>[2x]MEELQDDYEDMMEENLEQEEYEDPDIPESQMEEPAAHDTEATATDYHTTSHPGTHKVYVELQELVMDEKNQELRWMEAARWVQLEENLGENGAWGRPHLSHLTFWSLLELRRVFTKGTVLLDLQETSLAGVANQLLDRFIFEDQIRPQDREELLRALLLKHSHAGELEALGGVKPAVLTRSGDPSQPLLPQHSSLETQLFCEQGDGGTEGHSPSGILEKIPPDSEATLVLVGRADFLEQPVLGFVRLQEAAELEAVELPVPIRFLFVLLGPEAPHIDYTQLGRAAATLMSERVFRIDAYMAQSRGELLHSLEGFLDCSLVLPPTDAPSEQALLSLVPVQRELLRRRYQSSPAKPDSSFYKGLDLNGGPDDPLQQTGQLFGGLVRDIRRRYPYYLSDITDAFSPQVLAAVIFIYFAALSPAITFGGLLGEKTRN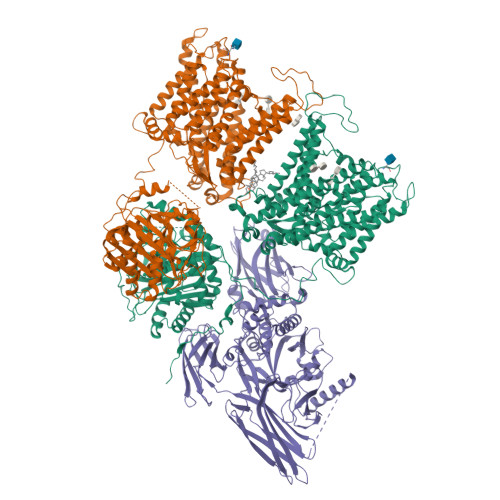QMGVSELLISTAVQGILFALLGAQPLLVVGFSGPLLVFEEAFFSFCETNGLEYIVGRVWIGFWLILLVVLVVAFEGSFLVRFISRYTQEIFSFLISLIFIYETFSKLIKIFQDHPLQKTYNYNVLMVPKPQGPLPNTALLSLVLMAGTFFFAMMLRKFKNSSYFPGKLRRVIGDFGVPISILIMVLVDFFIQDTYTQKLSVPDGFKVSNSSARGWVIHPLGLRSEFPIWMMFASALPALLVFILIFLESQITTLIVSKPERKMVKGSGFHLDLLLVVGMGGVAALFGMPWLSATTVRSVTHANALTVMGKASTPGAAAQIQEVKEQRISGLLVAVLVGLSILMEPILSRIPLAVLFGIFLYMGVTSLSGIQLFDRILLLFKPPKYHPDVPYVKRVKTWRMHLFTGIQIICLAVLWVVKSTPASLALPFVLILTVPLRRVLLPLIFRNVELQCLDADDAKATFDEEEGRDEYDEVAMPV;> MGQALGIKSCDFQAARNNEEHHTKALSSRRLFVRRGQPFTIILYFRAPVRAFLPALKKVALTAQTGEQPSKINRTQATFPISSLGDRKWWSAVVEERDAQSWTISVTTPADAVIGHYSLLLQVSGRKQLLLGQFTLLFNPWNREDAVFLKNEAQRMEYLLNQNGLIYLGTADCIQAESWDFGQFEGDVIDLSLRLLSKDKQVEKWSQPVHVARVLGALLHFLKEQRVLPTPQTQATQEGALLNKRRGSVPILRQWLTGRGRPVYDGQAWVLAAVACTVLRCLGIPARVVTTFASAQGTGGRLLIDEYYNEEGLQNGEGQRGRIWIFQTSTECWMTRPALPQGYDGWQILHPSAPNGGGVLGSCDLVPVRAVKEGTLGLTPAVSDLFAAINASCVVWKCCEDGTLELTDSNTKYVGNNISTKGVGSDRCEDITQNYKYPEGSLQEKEVLERVEKEKMEREKDNGIRPPSLETASPLYLLLKAPSSLPLRGDAQISVTLVNHSEQEKAVQLAIGVQAVHYNGVLAAKLWRKKLHLTLSANLEKIITIGLFFSNFERNPPENTFLRLTAMATHSESNLSCFAQEDIAICRPHLAIKMPEKAEQYQPLTASVSLQNSLDAPMEDCVISILGRGLIHRERSYRFRSVWPENTMCAKFQFTPTHVGLQRLTVEVDCNMFQNLTNYKSVTVVAPELSA>SGLVPAGSHMYLSMSISPETINVAGAQRMLSQKMAREALQLRLGAGDPKALAATIAQYERSAADLDAGNAERNVSRMGAPE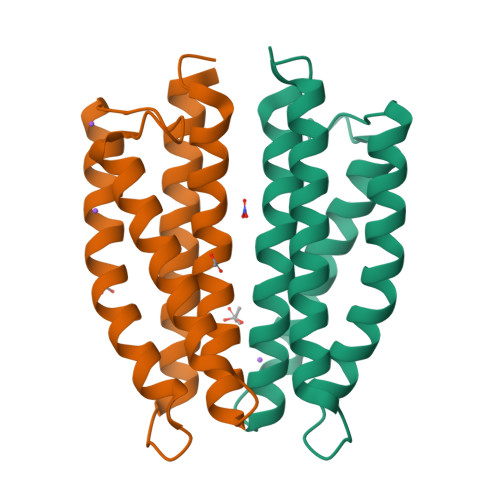IAAQRQKVAQIWGRYRAMLDQVAQPASQVDLRGFSQYSTELLGELNNLVSLMSARADSVQHTQMW[3x]>KESAAAKFERQHMDSSTSAASSSNYCNLMMCCRKMTQGKCKPVNTFVHESLADVKAVCSQKKVTCKDGQTNCYQSKSTMRITDCRETGSSKYPNCA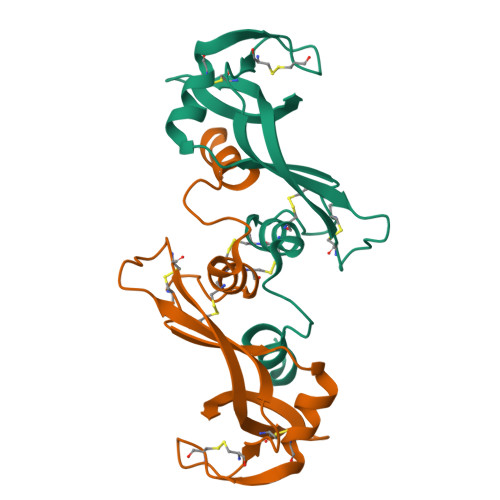YKTTQVEKHIIVACGGKPSVPVHFDASV[2x]>[4x]MARLDDLFIIHDTYVCLLSDHLLPNVIPVIQAPPQRVILLYTPNNKERVQRFRQATESVPTEIIEKQVHPYQ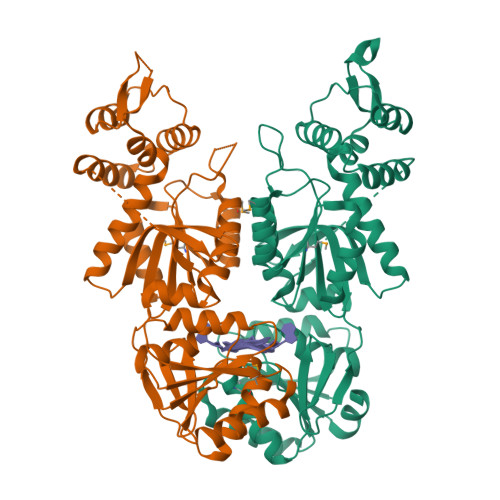YAQTQRICDEILEQFPNAILNVTGGTKIMALAAFDRFRHNHRPIIYVDSDSQRILYLHNGESERLGDPLTVKQYLACYGFKADNINRQDNLPKTWREVEDLFAQNSTKWQNQLGRLNWIAAQQQPIFTLQTGELQDLLLKANLIKPAEAKNAGFQFTSDQARQFINGGWFEHYVYSLLRQISAQYPIKNLTKNIEISNDSVSNELDVVFLYHNKLHVIECKTRHFTADGKINPMETIYKIDSVTNRVAGIKGKSMFASYYPLTQAAKKRCLNNSIYVSDQPSQLHHQLIKWINA Anaerobic ammonium oxidation (anammox) is a bacterial process in which ammonium and nitrite are combined into dinitrogen gas and water, yielding energy for the cell. As anammox bacteria express a large number of small c-type cytochromes, these have been proposed to perform the shuttling of electrons between the various parts of the metabolic machinery. Here, we present the structures and biochemical characterization of two of these proteins from the anammox model organism Kuenenia stuttgartiensis: Kustc0562 and highly homologous Kustc0563, which show relatively high transcription levels. Kustc0562 and Kustc0563 share 37% sequence identity after cleavage of the signal sequence and display a typical type-I cytochrome c fold.

In the crystal structure of Kustc0563, the heme iron is proximally coordinated by His47 and distally by Met91; in Kustc0562, the iron is proximally coordinated by the homologous His51, but the distal ligand is an imidazole molecule, presumably from the crystallization solution. Met94, the residue in Kustc0562 homologous to the distal Met in Kustc0563, has moved toward the side of the heme with the propionate groups to make space for imidazole, and a part of the loop containing this residue shows a different conformation than that in Kustc0563. The structures of Kustc0562 and Kustc0563 are highly similar, the main difference in the crystal structures being the presence of an axial imidazole ligand in the Kustc0562 structure, with an Fe–N distance of 2.1 Å. Given the high concentration of imidazole (100 mM) in the crystallization experiment, we believe this to be a crystallization artifact in which the “true” distal ligand, Met94, is displaced by imidazole. Indeed, when oxidized Kustc0562 was exposed in solution to the same concentration of imidazole as used in crystallization, a shift of the Soret band maximum from 411 to 406 nm accompanied by the disappearance of a charge-transfer band at 690 nm indicated a ligand exchange of methionine to imidazole. These spectral changes were reversed upon removal of imidazole. Spectropotentiometry revealed that Kustc0562 and Kustc0563 have redox potentials of +244 and +268 mV versus standard hydrogen electrode (SHE), respectively. Strikingly, however, despite the structural and electrochemical similarities between Kustc0562 and Kustc0563, only marginal activity could be detected when Kustc0562 was used as the electron acceptor. In contrast, despite the strong sequence similarity between the two proteins, the corresponding surface on Kustc0562 displays a pronounced positive charge, which would make interactions with the proposed binding site on the HAO surface electrostatically unfavorable. The striking contrast in electrostatics around the interaction sites on Kustc0562 and Kustc0563 provides an attractive explanation for this difference.

> EEKAIDARNLFEYHCAKCHGLTGEANKRGKALKAPDLCDPGWQNSKTDKEILYSITNGKNKMPAWNERLTPEEIEALARYVRKLSKKQR N-{3-[(4-aminobutyl)amino]propyl}acetamide | 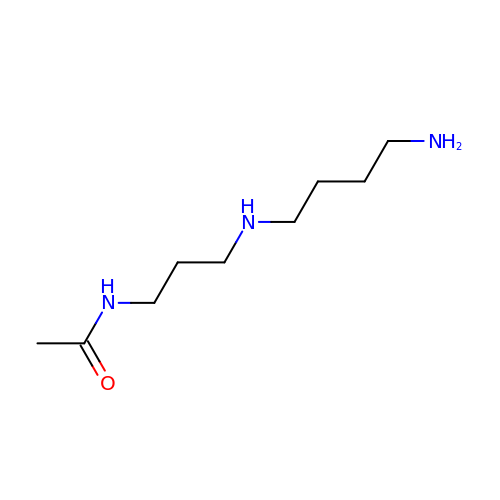C9 H21 N3 O | MQTAVJHICJWXBR-UHFFFAOYSA-N> FKVLQEPTCVSDYMSISTCEWKMNGPTNCSTELRLLYQLVFLLSEAHTCIPENNGGAGCVCHLLMDDVVSADNYTLDLWAGQQLLWKGSFKPSEHVKPRAPGNLTVHTNVSDTLLLTWSNPYPPDNYLYNHLTYAVNIWSENDPADFRIYNVTYLEPSLRIAASTLKSGISYRARVRAWAQAYNTTW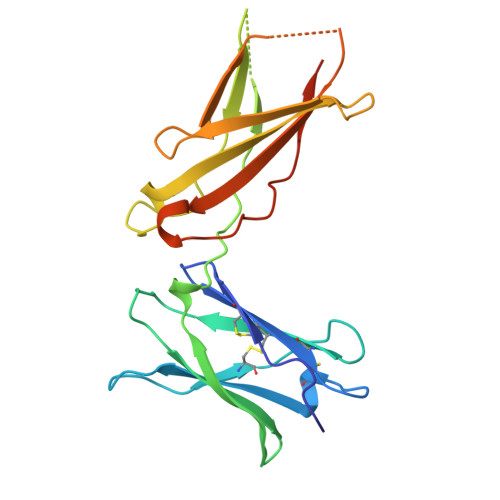SEWSPSTKWHNSYREPFEQH> AL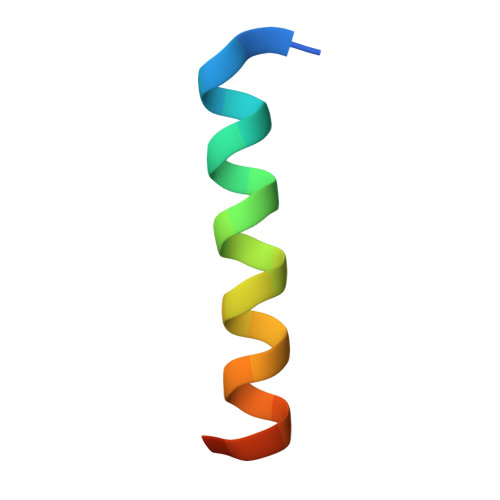WAAKKYGQQLRRMSDEFDKGQMKR>VTGDTDQPIHIESDQQSLDMQGNVVTFTGNVIVTQGTIKINADKVVVTRPGGEQGKEVIDGYGKPATFYQMQDNGKPVEGHAS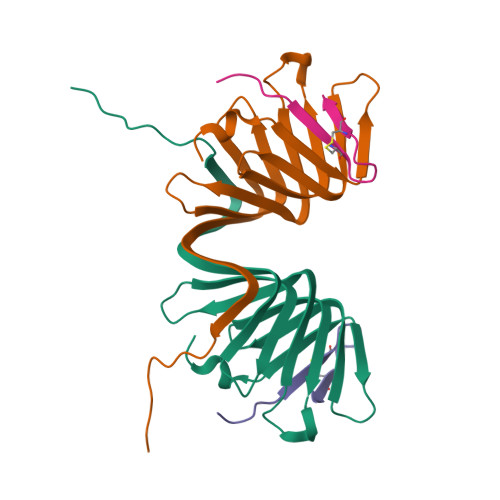QMHYELAKDFVVLTGNAYLQQVDSNIKGDKITYLVKEQKMQAFSDKGKR[2x];>[2x]GSKKPVPIIYCNRRTGKCQRM> MGGYLKVKMLSNEFQVPMRDSMLLSELKQLITQKIQVPAFRQRLLVQGSNEVLQDGVPLAHQGLRSGSEVVLVVQSCDRPLSILVRND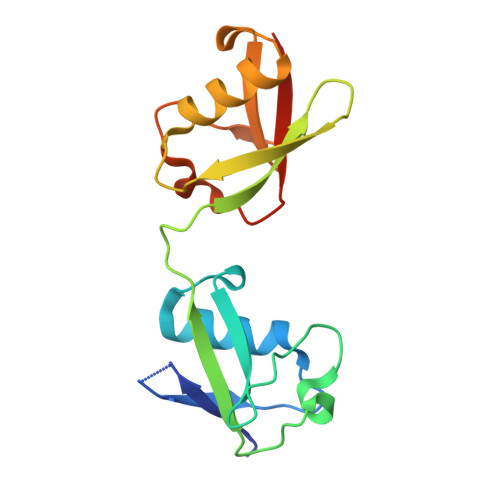RGNNRAYEVQLTQKVARLKEQVAERESTNVDQFWLSFQGQPLDDEKQLGEYDLTPHCTVQMNLRLRGG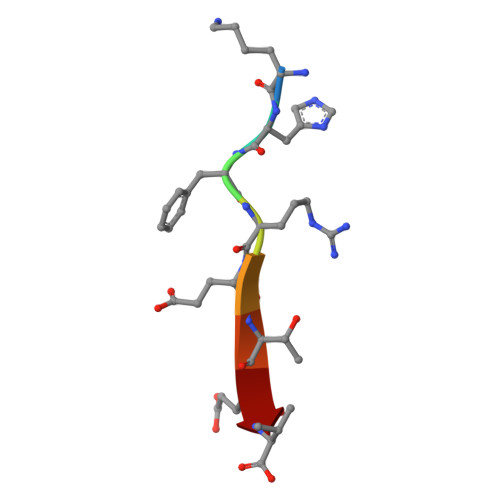> KHFRETEV> MIWTGLLVGFLFGIVLQRGRICFNSAFRDVLLFKDNYLFKLAVFTLALEMILFVLLSQVGLMQMNPKPLNLVGNIIGGFVFGLGMVLAGGAASGVTYRVGEGLTTAWFAALFYGLGAYATKSGAFSWWLSWVGQFKSPLSVEESAYYVKGAGPTISSVLGLNPWIPALVIAALFILWAFGTKTTSRETKFNWKIASVCL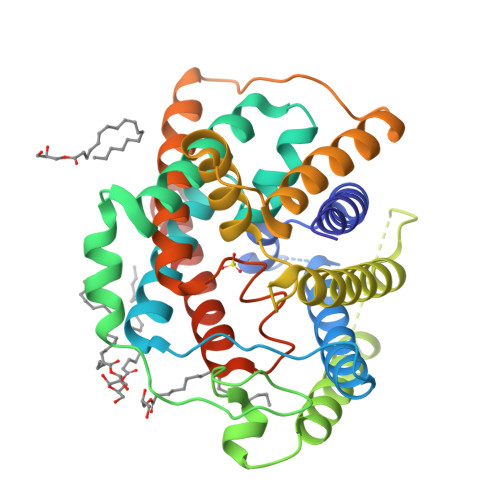ALVAGLGFITSTLSGRKYGLGITGGWINLFQGFLTNSPLNWEGLEIVGIILGAGVAAAVAGEFKLRMPKNPVTYLQVGIGGLLMGIGAVTAGGCNIGHFLTGVPQLALSSWLASIFFILGNWTMAWILFLESSGENLYFQ>[2x]MSLKIVIIGASFAGISAAIASRKKYPQAEISLIDKQATVGYLSGGLSAYFNHTINELHEARYITEEELRRQKIQLLLNREVVAMDVENQLIAWTRKEEQQWYSYDKLILATGASQFSTQIRGSQTEKLLKYKFLSGALAAVPLLENSQTVAVIGAGPIGMEAIDFLVKMKKTVHVFESLENLLPKYFDKEMVAEVQKSLEKQAVIFHFEETVLGIEETANGIVLETSEQEIS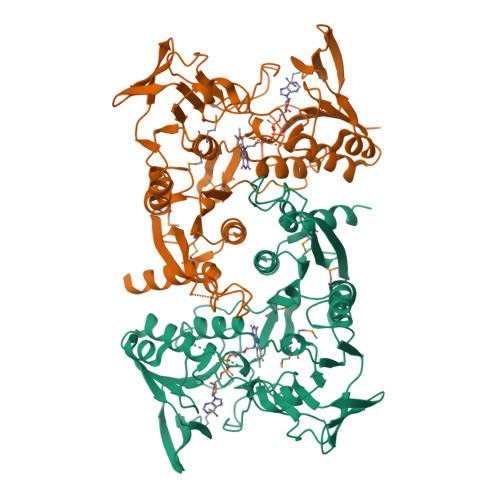CDSGIFALNLHPQLAYLDKKIQRNLDQTIAVDAYLQTSVPNVFAIGDCISVMNEPVAETFYAPLVNNAVRTGLVVANNLEEKTHRFIGSLRTMGTKVGDYYLASTGLTETEGLFFPQTLASIIVRQPAPPLQHGTEILGKLIYDKVTQRVLGAQLCSKNNCLEKINTLALSIQTGQTLTDLLQKDYFYQPSLTNIYDITNLMGASAYWRENDEGHHHHHH> GSHTPDESFLCYQPDQVCAFICRGAAPLPSEGECNPHPT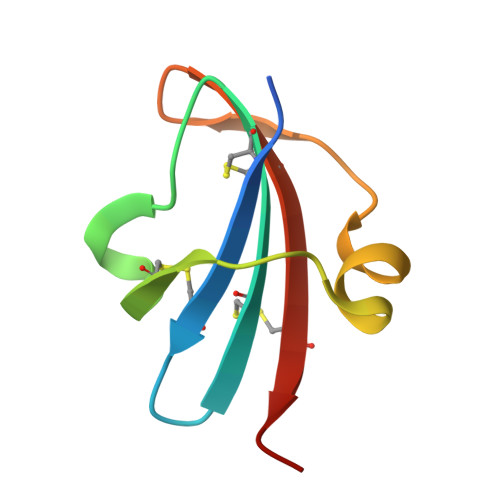APWAREGAVEWVPYSTGQCRTTCIPYVE>MYYLGKELQKRSEELSRGF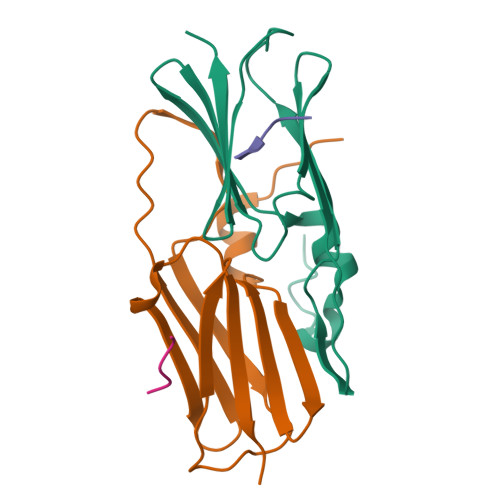YELVYPPVDMYEEGGYLVVVADLAGFNKEKIKARVSGQNELIIEAEREITEPGVKYLTQRPKYVRKVIRLPYNVAKDAEISGKYENGVLTIRIPIA[14x];>[9x]VIKIE> MAHHHHHHVDDDDKMSL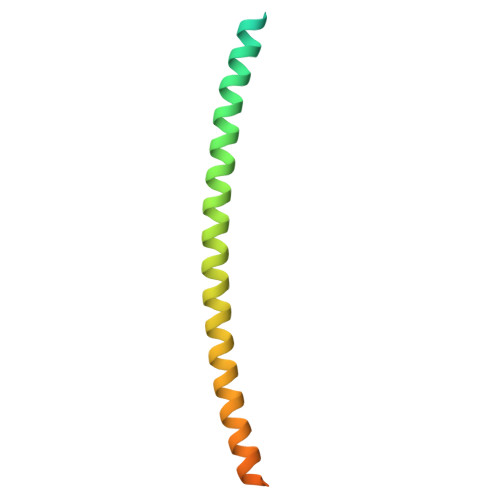LDAHIPQLIASHTAFAAKAGLMRHTIGQAEQQAMSAQAFHQGESAAAFQGAHARFVAAAAKVNTLLDIAQANLGEAAGTYVAADAAAASSYTGF> GSHMLSDEQMQIINSLVEA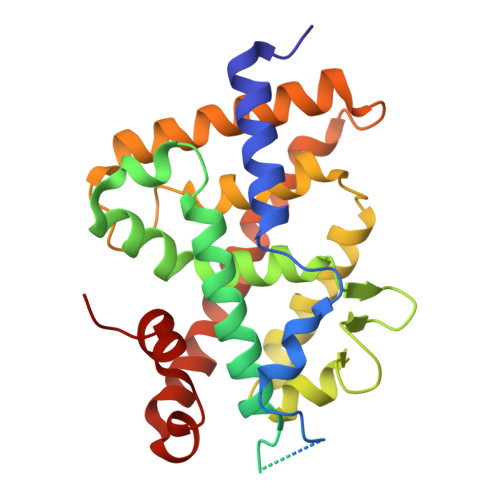HHKTYDDSYSDFVRFRPPVRVGPVTRSASRAASLHSLSDASSDSFNHSPESVDTKLNFSNLLMMYQDSGSPDSSEEDQQSRLSMLPHLADLVSYSIQKVIGFAKMIPGFRDLTAEDQIALLKSSAIEIIMLRSNQSFSLEDMSWSCGGPDFKYCINDVTKAGHTLELLEPLVKFQVGLKKLKLHEEEHVLLMAICLLSPDRPGVQDHVRIEALQDRLCDVLQAYIRIQHPGGRLLYAKMIQKLADLRSLNEEHSKQYRSLSFQPEHSMQLTPLVLEVFGSEVS[[(2~{R},3~{S},4~{R},5~{R})-5-[6-chloranyl-4-[[(1~{S})-1-(4-fluorophenyl)ethyl]amino]pyrazolo[3,4-b]pyridin-1-yl]-3,4-bis(oxidanyl)oxolan-2-yl]methoxy-oxidanyl-phosphoryl]methylphosphonic acid | C20 H24 Cl F N4 O9 P2 | 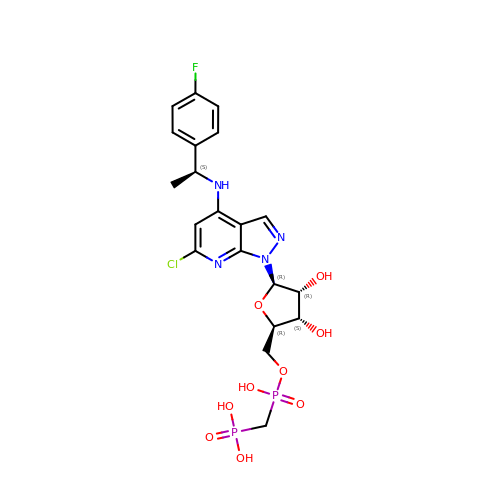ZOJVDXWVVGFWSE-KCVUFLITSA-N> K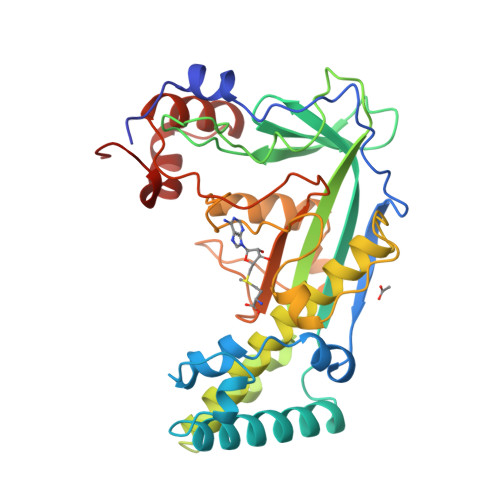KPRTPPVTLEAARDNDFAFDWQAYTPPVAHRLGVQEVEASIETLRNYIDWTPFFMTWSLAGKYPRILEDEVVGVEAQRLFKDANDMLDKLSAEKTLNPRGVVGLFPANRVGDDIEIYRDETRTHVINVSHHLRQQTEKTGFANYCLADFVAPKLSGKADYIGAFAVTGGLEEDALADAFEAQHDDYNKIMVKALADRLAEAFAEYLHERVRKVYWGYAPNENLSNEELIRENYQGIRPAPGYPACPEHTEKATIWELLEVEKHTGMKLTESFAMWPGASVSGWYFSHPDSKYYAVAQIQRDQVEDYARRKGMSVTEVERWLAPNLGYDAD> GSGHKSSPCDTNWRYYGDSCYGFFRHNLTWEESKQYCTDMNATLLKIDNRNIVEYIKARTHLIRWVGLSRQKSNEVWK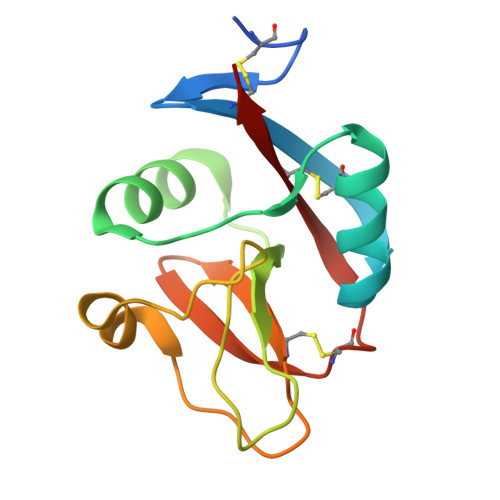WEDGSVISENMFEFLEDGKGNMNCAYFHNGKMHPTFCENKHYLMCERKAG>GPAVPRMDTTIDGFADSYEISSTSFVATDNTDSSIVYLAAEQVLTGPDVSALQLLSNSFESVFDSPDDFYSDAKLVLSDGREVSFHRCVLSARSSFFKSALAAAKKEKDSNNTAAVKLELKEIAKDYEVGFDSVVTVLAYVYSSRVRPPPKGVSECADENCCHVACRPAVDFMLEVLYLAFIFKIPELITLYQRHLLDVVDKVVIEDTLVILKLANICGKACMKLLDRCKEIIVKSNVDMVSLEKSLPEELVKEIIDRRKELGLEVPKVKKHVSNVHKALDSDDIELVKLLLKEDHTNLDDACALHFAVAYCNVKTATDLLKLDLADVNHRNPRGYTVLHVAAMRKEPQLILSLLEKGASASEATLEGRTALMIAKQATMAVECNNIPEQCKHSLKGRLCVEILEQEDKREQIPRDVPPSFAVAADELKMTLLDLENRVALAQRLFPTEAQAAMEIAEMKGTCEFIVTSLEPDRLTGTKRTSPGVKIAPFRILEEHQSRLKALSKTVELGKRFFPRCSAVLDQIMNCEDLTQLACGEDDTAEKRLQKKQRYMEIQETLKKAFSEDNLELGNSSLTDSTSSTSKSTGGKRSNRKLSHRRRGGWSHPQFER[2x];>GPANNDQDEDRINDKMKRRLAQNREAARKSRLRKKAHVQQLEESRLKLSQLEQELVRARQQGLCVRNSSDTSYLGPAGNMNSGIAAFEMEYTHWLEEQNRRVSEIRTALQAHIGDIELKMLVDSCLNHYANLFRMKADAAKADVFFLMSGMWRTSTERFFQWIGGFRPSELLNVVMPYVEPLTDQQLLEVRNLQQSSQ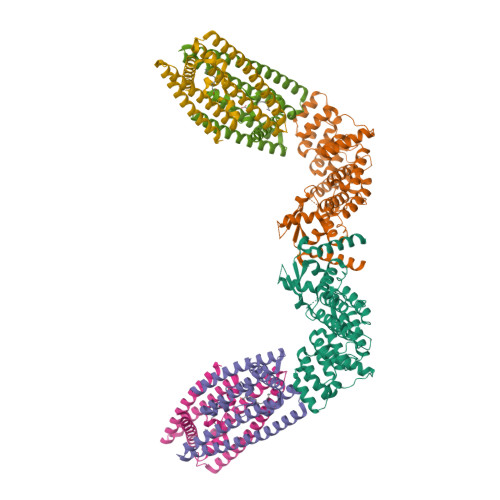QAEEALSQGLDKLQQGLVESIAIQIKVVESVNHGAPMASAMENLQALESFVNQADHLRQQTLQQMSKILTTRQAARGLLALGEYFHRLRALSSLWAARPREHTGGDYKDDDDKSSGYPYDVPDYA[4x]> GQPPLVPPRKEK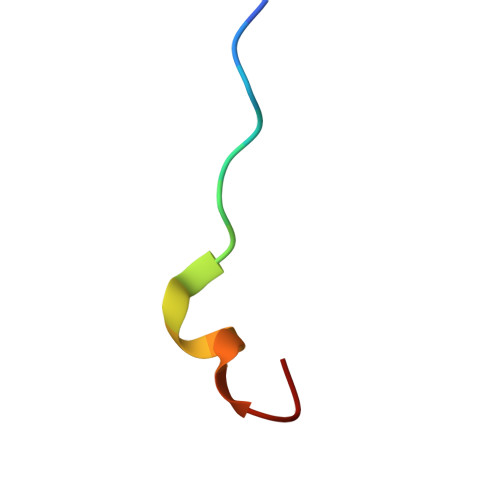MRGK>MGSSHHHHHHSQDPKRPMDTEEAEELVRQWENVKAEALGPTHQVYSLSEVLDESMLVQWQTLAQTAEAKSCYWRFVL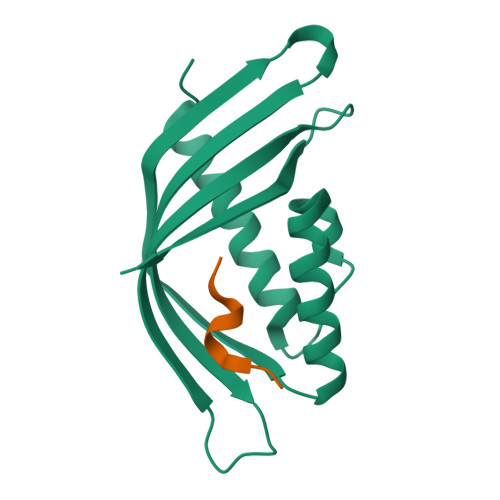LHLEVLQAHIFEDGIAGEAAEIEALLEEAAELVDESQPKNAKYYSTYKIRYILKKQEDGLWKFCQSDIQIQK[4x];>[4x]DHLDVMMARG> DDETGKELVLALYDYQEKSPREVTMKKGDILTLLNST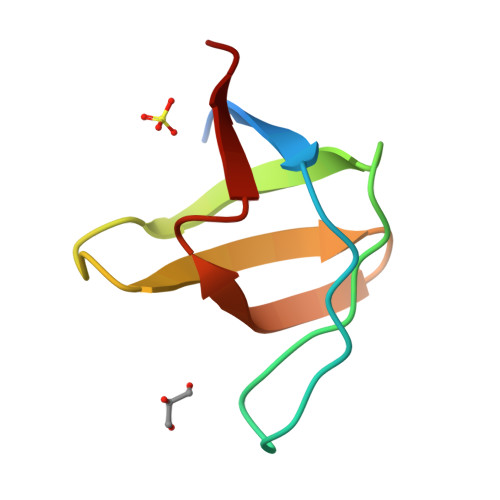NKDWWKVEVGDRQGFVPAAYVKKLD>MELENIVANTVLLKAREGGGGNRKGKSKKWRQMLQFPHISQCEELRLSLERDYHSLCERNPIGRLLFREFCATRPELSRCVAFLDGVAEYEVTPDDKRKACGRNLTQNFLSHTGPDLIPEVPRQLVTNCTQRLEQGPCKDLFQELTRLTHEYLSVAPFADYLDSIYFNRFLQWKWLERQPVTKNTFRQYRVLGKGGFGEVCACQVRATGKMYACKKLEKKRIKKRKGEAMALNEKQILEKVNSRFVVSLA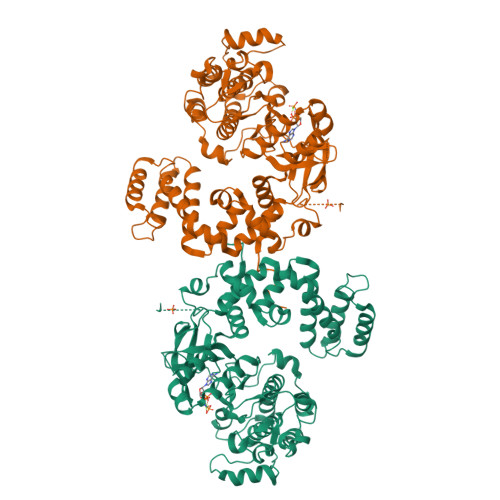YAYETKDALCLVLTLMNGGDLKFHIYHMGQAGFPEARAVFYAAEICCGLEDLHRERIVYRDLKPENILLDDHGHIRISDLGLAVHVPEGQTIKGRVGTVGYMAPEVVKNERYTFSPDWWALGCLLYEMIAGQSPFQQRKKKIKREEVERLVKEVPEEYSERFSPQARSLCSQLLCKDPAERLGCRGGSAREVKEHPLFKKLNFKRLGAGMLEPPFKPDPQAIYCKDVLDIEQFSTVKGVELEPTDQDFYQKFATGSVPIPWQNEMVETECFQELNVFGLDGSVPPDLDWKGQPPAPPKKGLLQRLFSRQDSSGNSSDSEEELPTRL[2x]>[6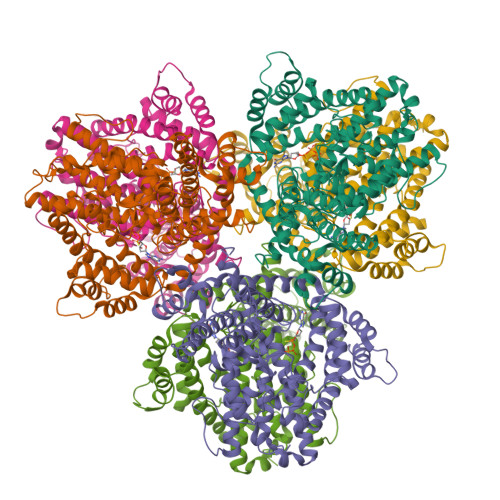x]MAQIDFRKKINWHRRYRSPQGVKTEHEILRIFESDRGRIINSPAIRRLQQKTQVFPLERNAAVRTRLTHSMEVQQVGRYIAKEILSRLKELKLLEAYGLDELTGPFESIVEMSCLMHDIGNPPFGHFGEAAINDWFRQRLHPEDAESQPLTDDRCSVAALRLRDGEEPLNELRRKIRQDLCHFEGNAQGIRLVHTLMRMNLTWAQVGGILKYTRPAWWRGETPETHHYLMKKPGYYLSEEAYIARLRKELNLALYSRFPLTWIMEAADDISYCVADLEDAVEKRIFTVEQLYHHLHEAWGQHEKGSLFSLVVENAWEKSRSNSLSRSTEDQFFMYLRVNTLNKLVPYAAQRFIDNLPAIFAGTFNHALLEDASECSDLLKLYKNVAVKHVFSHPDVERLELQGYRVISGLLEIYRPLLSLSLSDFTELVEKERVKRFPIESRLFHKLSTRHRLAYVEAVSKLPSDSPEFPLWEYYYRCRLLQDYISGMTDLYAWDEYRRLMAVEQ> GGCUUAUCAAGAGAGGGGGAGCGACUGGCGCGAAGAAC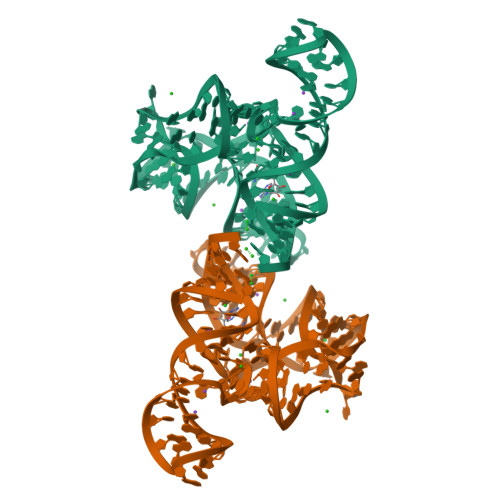CCCGGCAACCAGAAAUGGUGCCAAUUCCUGCAGCGGAAACGUUGAAAGAUGAGCCG> MEKYNPHAIEAKWQRFWEEKGFMKAKDLPGGRGKQYVLVMFPYPSGDLHMGHLKNYTMGDVLARFRRMQGYEVLHPMGWDAFGLPAENAALKFGVHPKDWTYANIRQAKESLRLMGILYDWDREVTTCEPEYYRWNQWIFLKMWEKGLAYRAKGLVNWCPKCQTVLANEQVVEGRCWRHEDTPVEKRELEQWYLRITAYAERLLKDLEGLNWPEKVKAMQRAWIGRSEGAEILFPVEGKEVRIPVFTTRPDTLFGATFLVLAPEHPLTLELAAPEKREEVLAYVEAAKRKTEIERQAEGREKTGVFLGAYALNPATGERIPIWTADYVLFGYGTGAIMAVPAHDQRDYEFARKFGLPIKKVIERPGEPLPEPLERAYEEPGIMVNSGPFDGTESEEGKRKVIAWLEEKGLGKGRVTYRLRDWLISRQRYWGTPIPMVHCEACGVVPVPEEE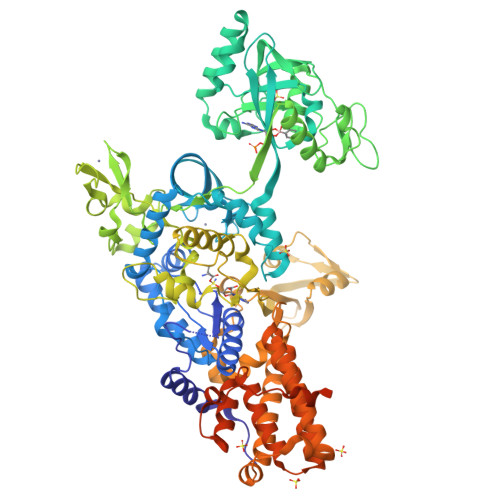LPVLLPDLKDVEDIRPKGKSPLEAHPEFYETTCPKCGGPAKRDTDTMDTFFDSSWYYLRYTDPHNDRLPFDPEKANAWMPVDQYIGGVEHAVLHLLYSRFFTKFLHDLGMVKVEEPFQGLFTQGMVLAWTDFGPVEVEGSVVRLPEPTRIRLEIPESALSLEDVRKMGAELRPHEDGTLHLWKPAVMSKSKGNGVMVGPFVKEQGADIARITILFAAPPENEMVWTEEGVQGAWRFLNRIYRRVAEDREALLETSGVFQAEALEGKDRELYGKLHETLKKVTEDLEALRFNTAIAALMEFLNALYEYRKDRPVTPVYRTAIRYYLQMLFPFAPHLAEELWHWFWPDSLFEAGWPELDEKALEKDVVEVAVQVNGAVAGTIHIPKDAPLEVARAEALKVRNVRAHLEGKEVVKEIYVPGKILNLVVRG>[2x]GPQDPDKRRKTLVIIEKTYSLLLDVEDYERRYLLSLEEE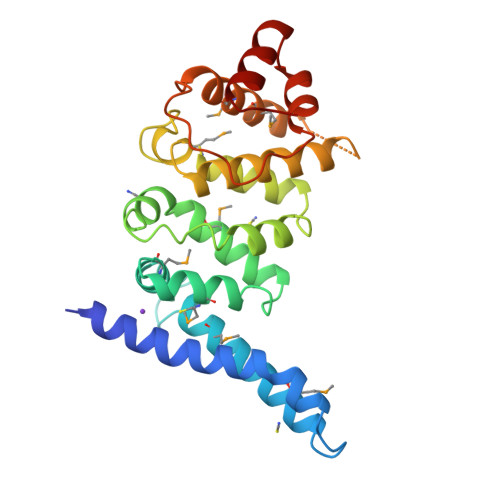RPALMDDRKHKICSMYDNLRGKLPGQERPSDDHFVQIMCIRKGKRMVARILPFLSTEQAADILMTTARNLPFLIKKDAQDEVLPCLLSPFSLLLYHLPSVSITSLLRQLMNLPGSPHLTAVLQNKFGLSLLLILLSRGEDLQSSDPATESTQNNQWTEVMFMATRELLRIPQAALAKPISIPTNLVSLFSRYVDRQKLNLLETKLQLVQ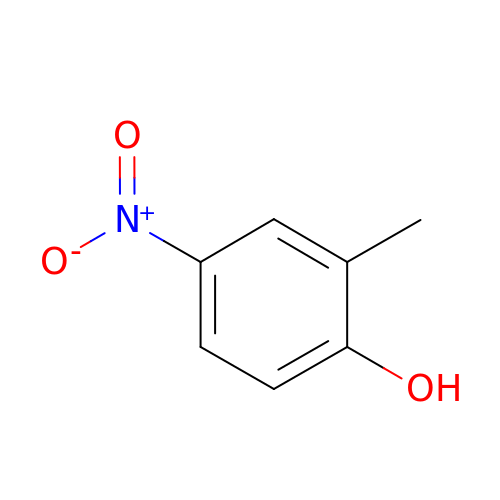2-methyl-4-nitrophenol | C7 H7 N O3 | KDQPMQNHVQVVMR-UHFFFAOYSA-N> LYPIAVLIDELRNEDVQLRLNSIKKLSTIALALGVERTRSELLPFLTDTIYDEDEVLLALAEQLGTFTTLVGGPEYVHCLLPPLESLATVEETVVRDKAVESLRAISHEHSPSDLEAHFVPLVKRLAGGDWFTSRTSACGLFSV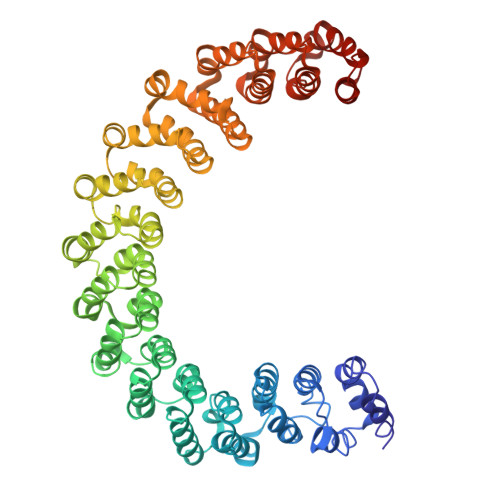CYPRVSSAVKAELRQYFRNLCSDDTPMVRRAAASKLGEFAKVLELDNVKSEIIPMFSNLASDEQDSVRLLAVEACVNIAQLLPQEDLEALVMPTLRQAAEDKSWRVRYMVADKFTELQKAVGPEITKTDLVPAFQNLMKDCEAEVRAAASHKVKEFCENLSADCRENVIMSQILPCIKELVSDANQHVKSALASVIMGLSPILGKDNTIEHLLPLFLAQLKDECPEVRLNIISNLDCVNEVIGIRQLSQSLLPAIVELAEDAKWRVRLAIIEYMPLLAGQLGVEFFDEKLNSLCMAWLVDHVYAIREAATSNLKKLVEKFGKEWAHATIIPKVLAMSGDPNYLHRMTTLFCINVLSEVCGQDITTKHMLPTVLRMAGDPVANVRFNVAKSLQKIGPILDNSTLQSEVKPILEKLTQDQDVDVKYFAQEALTVLSLA> APNTSGFNLRGTTQVPTELQKLLLESSDPYGPLARSIRQQLRLNNVTIVDDAMRKDIPTLRIIGSSESQETVSIFRNGVAAENQLVLHVQAQVLIPGHDIYPLQVNVFRTFFDNPLTALAKEAEAEVLRQEMREQAAQQLVRQLLTVHAAEVKNTQKNGDKP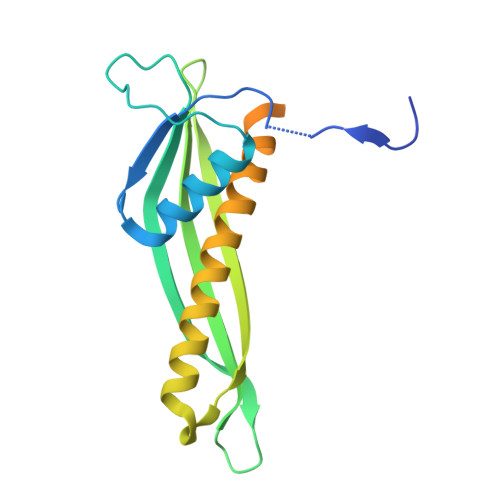VSDANAAQGSTPTAVNETTLGEPAVSTSAKHHHHHH> GPGEASMLRDKINFLNIEREKEKNIQAVKVNELQVKHLQELA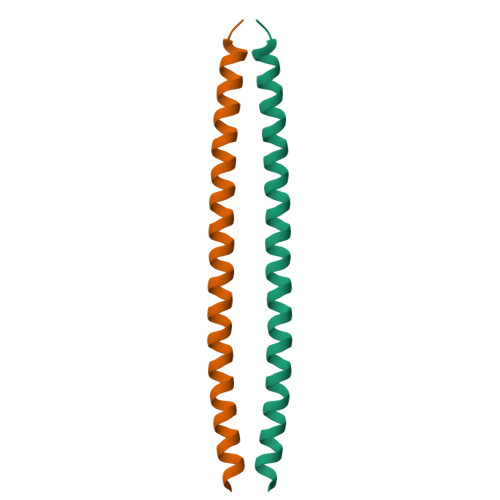KLKQELQKLEDEKKFLQMEARGKS> SQFVGSDGMGGDAAAPGAAGTQAELPHRRFEY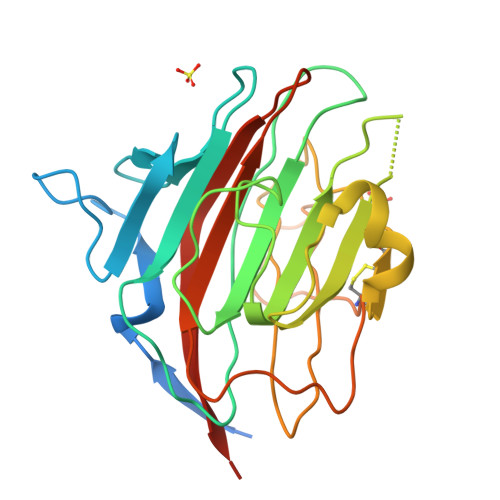KYSFKGPHLVQSDGTVPFWAHAGNAIPSADQIRIAPSLKSQRGSVWTKTKAAFENWEVEVTFRVTGRGRIGADGLAIWYTENQGLDGPVFGSADMWNGVGIFFDSFDNDGKKNNPAIVVVGNNGQINYDHQNDGATQALASCQRDFRNKPYPVRAKITYYQKTLTVMINNGFTPDKNDYEFCAKVENMVIPTQGHFGISAATGGLADDHDVLSFLTFQLTEPGKEPPT>[2x]GSHMDSQFYSVQVADSTFTVLKRYQQLKPIGSGAQGIVCAAFDTVLGINVAVKKLSRPFQNQTHAKRAYRELVLLKCVNHKNIISLLNVFTPQKTLEEFQDVYLVMELMDANLCQVIHMELDHERMSYLLYQMLCGIKHLHSAGIIHRDLKPSNIVVKSDCTLKILDFGLARTASTNFMMTPYVVTRYYRAPEVILGMGYKENVDIWSVGCIMGELVKGSVIFQGTDHIDQWNKVI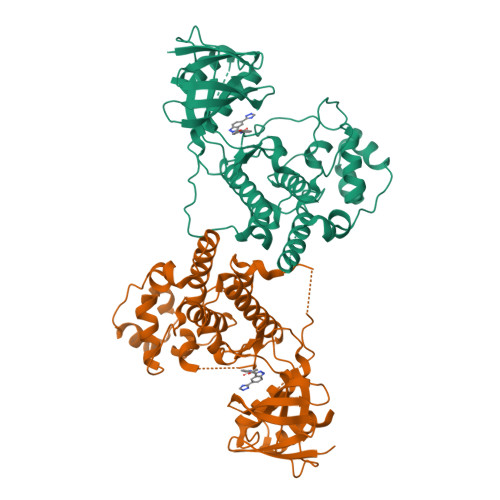EQLGTPSAEFMAALQPTVRNYVENRPAYPGIAFEELFPDWIFPSESERDKIKTSQARDLLSKMLVIDPDKRISVDEALRHPYITVWYDPAEAEAPPPQIYDAQLEEREHAIEEWKELIYKEVMD> SMEEVGKGGQSAKFVTYSTSEPAKLFGEAGRRSHFRARVLEATLSPLEKAIFDVPIEEWLTVDRSKFSGWRCAVPHPVTADELKPVDSSHDILRHIALYNGPVTDLQLDAIVNAANKTCLGGKGVDGAIHAAAGPLLVRECATFKGCDTGQCRLTKGYNLPARYVLHTVGPIGERPEELRSCYRSILSLAHRNRLRSIGFCCVSTGVYGYPLIPATRIAVDETIEYLKQHFSAFDLCCFACFKLEEYNAYTDCLRAWLGTAPNASTDQ

We named these proteins as Trypanosoma brucei MacroD-like protein (TbMDO) and Trypanosoma cruzi MacroD-like protein (TcMDO). We show that the trypanosomatid MacroD1/MacroD2 homologues are hydrolyzing both protein-linked ADP-ribose and free O-acetyl-ADP-ribose. The macrodomain fold (starting from residues 99 and 92 in TbMDO and TcMDO, respectively) is well-conserved between the human MacroD proteins and consists of a central mostly parallel six-stranded β-sheet surrounded by five α-helices. Active site of the macrodomains is located at the C-terminal edge of the β-sheet and is lined by N-terminal ends of four α-helices.

Crystal structures of TbMDO were determined to 1.95 Å and 1.2 Å resolution (for crystal form 1 and 2, respectively) and crystal structure of TcMDO to 2.0 Å resolution. Structures of TbMDO and TcMDO comprise residues from 11–261 and 13–257, respectively and share a highly conserved structure (RMSD 0.84 Å). The N-terminus of TbMDO and TcMDO also pack differently in the crystal. While the N-terminus of the TbMDO folds back to the core and extends the β-sheet, the N-terminus of the TcMDO packs to the precisely same site but in the neighboring molecule in the crystal. No complex of ADP-ribose with TcMDO could be acquired but comparing the TbMDO-ADP-ribose complex with TcMDO revealed that a loop aligning the distal ribose binding pocket adopts an open conformation, indicating that the ADP-ribose binding pocket at this region is not preformed in TcMDO. The observed open conformation is unlikely a crystal packing artefact, as there are no major constrictions caused by packing at this region of the crystal lattice. In addition, an identical conformation for the loop is observed in the apo-structure of human MacroD1. The larger enthalpy drop in TcMDO could be due to the open conformation of the active site. In the open conformation, the loop near the distal ribose is unable to interact with the phosphates of ADP and might explain the enthalpy change. Also TcMDO contains proline in this position indicating similar binding mode of the adenine moiety as observed in TbMDO.>MAFDGSIKSLLQGVSQQVPRERLDGQVSVQLNRLSDVVNGNRRRPGARYLADVPTTSQYDDHVFASYVDVQDTANHVIINTETGQLLVISEDFSTTLHNSTQQYLVASAASAIQTATLRGDLYIANTEKAPTKVFGSTTQQDPTKAGFYFVRTPALQKDYDITLSNSTGTYTYTYRTPTGTGTGDADLAKPSYIISDLLAKINAQTGTHGITATAYDAYMFLSSNTVSLSVTTNAGSTYATGSNQSRVSVVSDLPARLPAVGNGASVAVGTTERNFVWYQYDSATSVWKEAGAYGSPTGFSNMPIRISLDGVYTVETPAYEGRLAGSDETNEDPGFIDNGVTGFGAYQGRLVILAGPEVCMSAAGNPLRWYRSTVTALLTDDPINIFSGAATSTNFRHCVQFNKDLLLFARSCQAVVPSSNAAITPQTAQIVITSGYTTDTLAQPGVVGRSVLYSMPRTEHFAGVLEIIPSNTTDSQYTSNDITAHIPRYLPGRIRSIVSSTTSNSSAFICTGDSRSLFIQDYLWSGDEKVQSAWHQWTLPYPIVCTWFVRDRVYIGMRDGTTILVVTIEPQAGNTIDSYVRPFSDVYLRVTITDRQFALPTRLRAAVGSGEGLFITFADTSMGGMWVGYESIDPTTYVVTTVRNVPDGEYFVGLRYTSVLSPTPPLVRDANGIVIGTYQSLLVRYELTLKDSGEFHAIITDSSRTLTDGNYSSLVYSSTELLPNNPTDASLGRTIIPVRAQAQDTVATFEANADTDLCILDIEYVLQYRARRKRI[6x];>MYSVQIAVSDGTLTRIALSIEYFEKDDITLYRNLELTPLVLGTDWQWDGDTHINLLTGIPVPVGSYITVRRNTDIDRAFNIYDGGAAFNRETLDENFKQMIYLAQEFTEGNGLTGLYFPLDMHGFQIKNLGEPTDPGDAVTKQYVDTANTAQNANFNASQQAQDQAVAASQAVQDNRLASLENTFVQATSSYPWYTVSTSTTDTFTPGFNFTKAAVYINGVCQTPDYSYIVVANQILLADPVPLGTMVFARLGEDIQNDDDFATTAQLSAVQANLQDEIDVTNTEVSNKASKGANSDISSLSGLTTPLSAAQGGTGNNTGNAATATVLATPRTIQTNLASTSAASFNGSANITPGVTGNLPVTNGG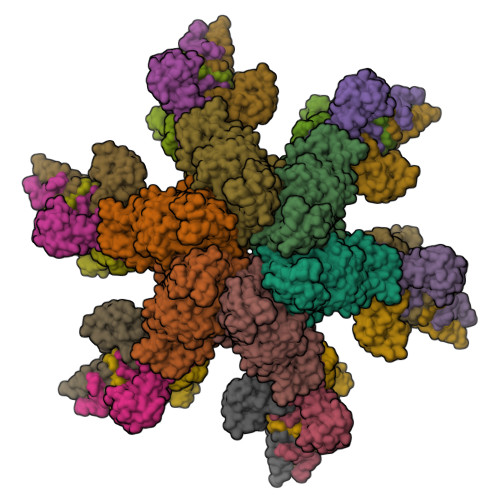TGAGSAPSARANLGAAMNGINNDISNLAALTGGITGLTTGTAAASGIVGEVASAASSSATNLVSGSVINIISLSLPAGDWELESAFQIINTGNVTALAFGVSTTTGVLPTPWYDVYSITTTIGSGTSNRQGMARRVLLSTTTTVYLVAQATFTGTATANGYVRARRVR[18x]>[2x]MKLKSFGVFGNPIKHSKSPLIHNACFLTFQKELRFLGHYHPILLPLESHIKSEFLHLGLSGANVTLPFKERAFQVCDKIKGIALECGAVNTLVLENDELVGYNTDALGFYLSLKQKNYQNALILGAGGSAKALACELKKQGLQVSVLNRSSRGLDFFQRLGCDCFMEPPKSAFDLIINATSASLHNELPLNKEVLKGYFKEGKLAYDLAAGFLTPFLSLAKELK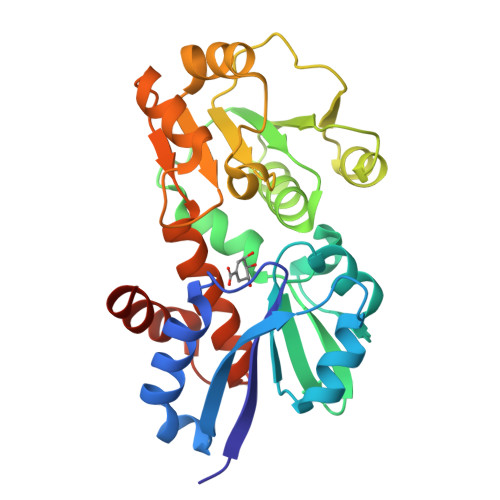TPFQDGKDMLIYQAALSFEKFSASQIPYSKAFEVMRSVFLEHHHHHH>VMFIDGKWINREDMDVINPYSLEVIKKIPALSREEAKEAIDTAEKYKEVMKNLPITKRYNILMNIAKQIKEKKEELAKILAIDAGKPIKQARVEVERSIGTFKLAAFYVKEHRDEVIPSDDRLIFTRREPVGIVGAITPFNFPLNLSAHKIAPAIATGNVIVHHPSSKAPLVCIELAKIIENALKKYNVPLGVYNLLTGAGEVVGDEIVVNEKVNMISFTGSSKVGELITKKAGFKKIALELGGVNPNIVLKDADLNKAVNALIKGSFIYAGQVCISVGMILVDESIADKFIEMFVNKAKVLNVGNPLDEKTDVGPLISVEHAEWVEKVVEKAIDEGGKLLLGGKRDKALFYPTILEVDRDNIL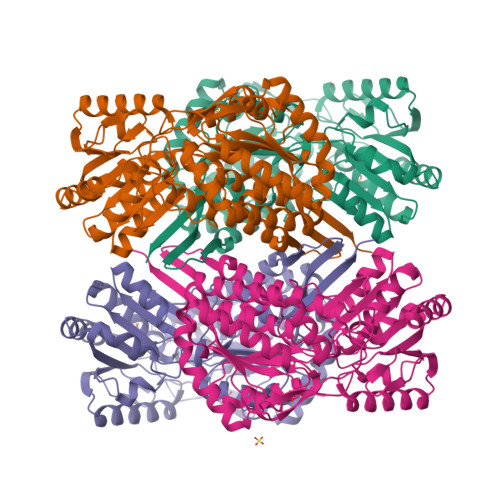CKTETFAPVIPIIRTNEEEMIDIANSTEYGLHSAIFTNDINKSLKFAENLEFGGVVINDSSLFRQDNMPFGGVKKSGLGREGVKYAMEEMSNIKTIIISKAENLYFQSHHHHHHWSHPQFEK[4x]> GSHMRTVSVEAIVEALVAEGALRPEEIA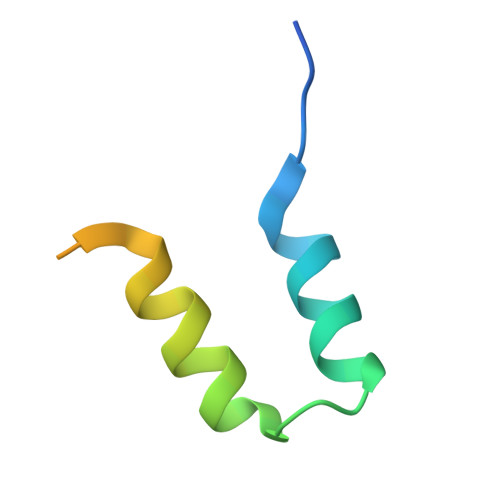DFVERITTLDIGTDIFEEQDEGDYWW> SGPINDTDANPRYKIPVEADFLFAYSTVPGYVSMRSPGRGSWFVQALCSILEEHG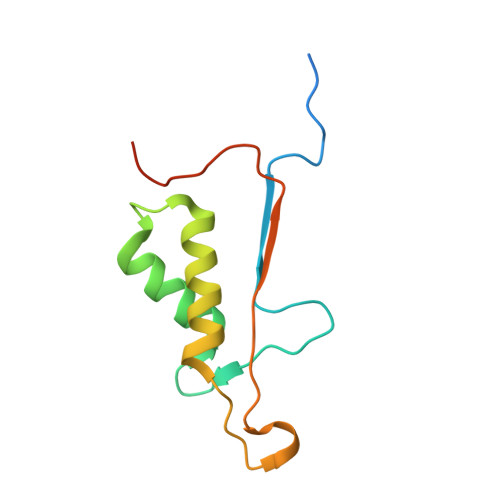KDLEIMQILTRVNDRVARHFESCSDDPHFHEKKQIPCVVSMLTKELYFSQLEHHHHHH> ADYQGKNVVIIGLGLTGLSCVDFFLARGVTPRVMDTRMTPPGLDKLPEAVERHTGSLNDEWLMAADLIVASPGIALAHPSLSAAADAGIEIVGDIELFCREAQAPIVAITGSNGKSTVTTLVGEMAKAAGVNVGVGGNIGLPALMLLDDECELYVLELSSFQLETTSSLQAVAATILNVTEDHMDRYPFGLQQYRAAKLRIYENAKVCVVNADDALTMPIRGADERCVSFGVNMGDYHLNHQQGETWLRVKGEKVLNVKEMKLSGQHNYTNALAALALADAAGLPRASSLKALTTFTGLPHRFEVVLEHNGVRWINDSKATNVGSTEAALNGLHVDGTLHLLLGGDGKSADFSPLARYLNGDNVRLYCFGRDGAQLAALRPEVAEQTETMEQAMRLLAPRVQPGDMVLLSPACASLDQFKNFEQRGNEFARLAKELG

MurD catalyzes the addition of D-glutamic acid to UDP-MurNAc-L-Ala, generating the dipeptide moiety L-Ala-D-Glu in almost all bacterial species. From a structural point of view, Mur ligases are three-domain enzymes that share a very well conserved ATP-binding site that harbors the Gly-X-X-Gly-Lys-Thr/Ser motif and display notable structural similarities in terms of domain arrangement. The N-terminal domain is involved in the binding of the UDP-precursor, the central domain in the binding of ATP, and the C-terminal domain in the binding of the amino acid or dipeptide. Crystal structures of Mur ligases reveal that MurC, MurD and MurF display at least two distinct conformations, namely ‘open’ and ‘closed’, with the position of C-terminal domain dictating the nature of the conformation.

We achieved this by solving two intermediate conformations of MurD which we named Intermediate Free MurD (i.e., intermediate conformation of ligand-free MurD) and Intermediate Bound MurD (i.e., intermediate conformation of MurD with ligands). In the solving of Intermediate Free MurD, 421 residues were refined. There is one minor region missing between residues Thr180─Tyr187 since it could not be traced in the electron density map. Notably, Lys198 is not carbamoylated as it is the case in open MurD structures. Superposition to open unbound MurD structure revealed that the new structure was clearly in a distinct conformation. Only Arg302 was found to be differently oriented so we focused on this residue because of its position in the hinge loop containing residues from Thr294 to Glu304. There is a difference in the orientation of Arg302 as well as its interactions, when compared to the previously solved closed conformations of MurD and additionally orientation of Arg302 in Intermediate Free MurD is different from all of the orientations found in the aforementioned structures of MurD, which contributes towards the intermediate conformation adopted by the protein. Thus, we were able to ‘trap’ an intermediate conformation of MurD that is not open despite the absence of ligands, nor closed in the presence of ligands. This suggests that it is not substrate recognition which causes MurD closure, as previously suggested, but that domain movement is an inherent feature of the enzyme that is independent of ligand binding.>[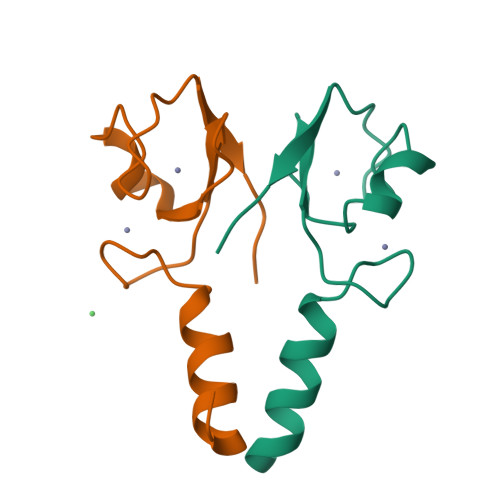2x]GPLGSTSLQKEISTEEQLRRLQEEKLCKICMDRNIAIVFVPCGHLVTCKQCAEAVDKCPMCYTVITFKQKIFMS> GPLGSLEPPLWHAEFTK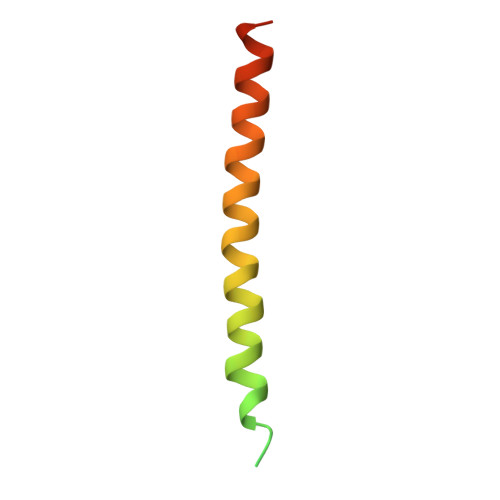EELVQKLSSTTKSADHLNGLLRETEATNAILMEQIKLLKSEIRRLERNQEREKS> TNKIKIGHVHMSGCTGCLVSLADNNLGLIKILDDYADLVYCLTLADVRHIPEMDVALVEGSVCLQDHESVEDIKETRKKSKIVVALGSCACYGNITRFSRGGQHNQPQHESYLPIGDLIDVDVYIPGCPPSPELIRNVAVMAYLLLEGNEEQKELAGKYLKPLMDLAKRGT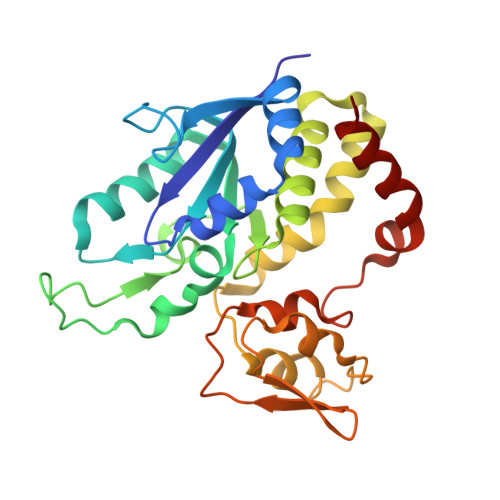SGCFCDLMYDVINQGLCMGCGTCAASCPVHAITLEFGKPQGERDLCIKCGSCYGACPRSFFNLDVISEFENISEIIAKALKD>MEGGPALFQSDMTFKIFID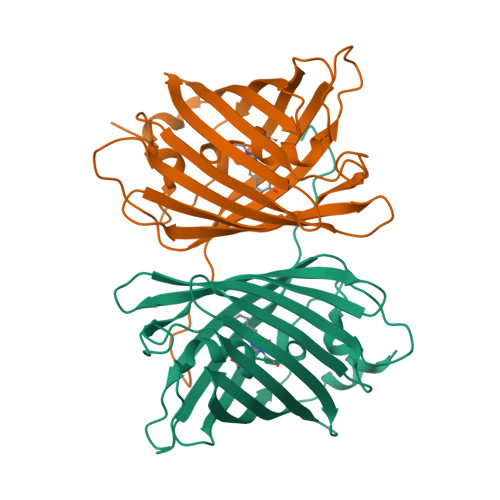GEVNGQKFTIVADGSSKFPHGDFNVHAVCETGKLPMSWKPICHLIQYGEPFFARYPDGISHFAQECFPEGLSIDRTVRFENDGTMTSHHTYELDDTCVVSRITVNCDGFQPDGPIMRDQLVDILPNETHMFPHGPNAVRQLAFIGFTTADGGLMMGHFDSKMTFNGSRAIEIPGPHFVTIITKQMRDTSDKRDHVCQREVAYAHSVPRITSAIGSDED[2x]> SESQEDIIRNIARHLAQVGDSMDRSIPP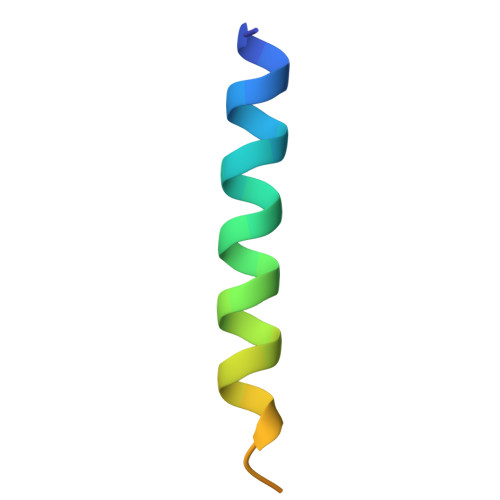GLVNGL> MPREIITLQLGQCGNQIGFEFWKQLCAEHGISPEGIVEEFATEGTDRKDVFFYQADDEHYIP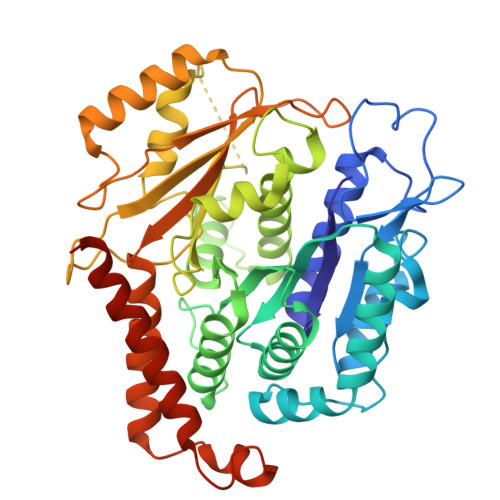RAVLLDLEPRVIHSILNSPYAKLYNPENIYLSEHGGGAGNNWASGFSQGEKIHEDIFDIIDREADGSDSLEGFVLCHSIAGGTGSGLGSYLLERLNDRYPKKLVQTYSVFPNQDEMSDVVVQPYNSLLTLKRLTQNADCVVVLDNTALNRIATDRLHIQNPSFSQINQLVSTIMSASTTTLRYPGYMNNDLIGLIASLIPTPRLHFLMTGYTPLTTDQSVASVRKTTVLDVMRRLLQPKNVMVSTGRDRQTNHCYIAILNIIQGEVDPTQVHKSLQRIRERKLANFIPWGPASIQVALSRKSPYLPSAHRVSGLMMANHTSISSLFESSCQQYDKLRKREAFLEQFRKEDIFKENFDELDRSREVVQELIDEYHAATRPDYISWGTQEQ3-chloro-5-({6-[2-(3,4-dihydroisoquinolin-2(1H)-yl)-2-oxoethyl]-3-(dimethylamino)-2-oxo-1,2-dihydropyridin-4-yl}oxy)benzonitrile | C25 H23 Cl 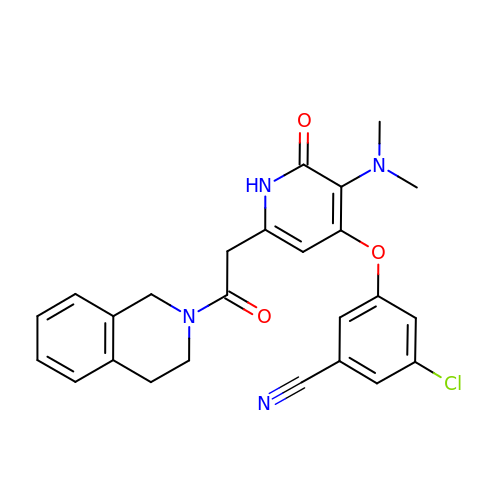N4 O3 | CLCCLHPVIUSCJF-UHFFFAOYSA-N KANAMYCIN C | C18 H36 N4 O11 | 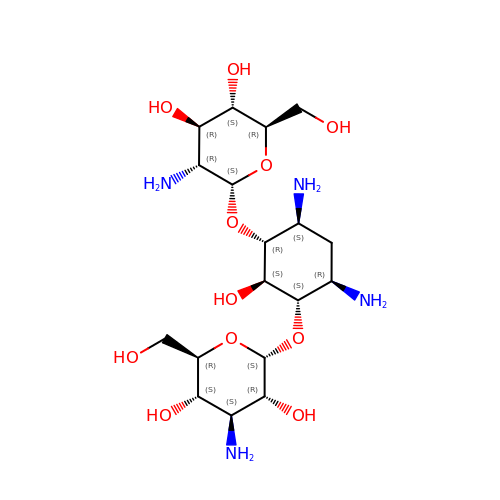WZDRWYJKESFZMB-FQSMHNGLSA-N> ALEEAPWPPPEGAFVGFVLSRK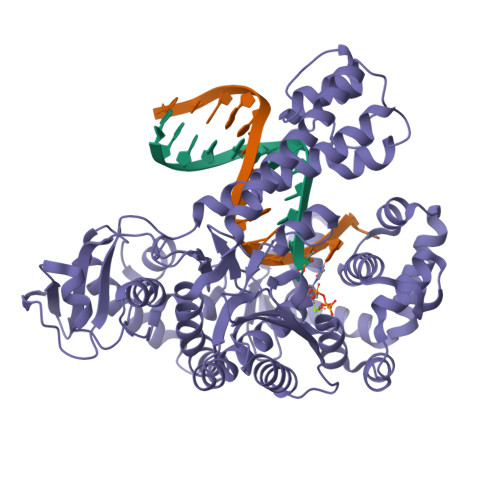EPMWADLLALAAARGGRVHRAPEPYKALRDLKEARGLLAKDLSVLALREGLGLPPGDDPMLLAYLLDPSNTTPEGVARRYGGEWTEEAGERAALSERLFANLWGRLEGEERLLWLYREVERPLSAVLAHMEATGVRLDVAYLRALSLEVAEEIARLEAEVFRLAGHPFNLNSRDQLERVLFDELGLPAIGKTEKTGKRSTSAAVLEALREAHPIVEKILQYRELTKLKSTYIDPLPDLIHPRTGRLHTRFNQTATATGRLSSSDPNLQNIPVRTPLGQRIRRAFIAEEGWLLVALDYSQIELRVLAHLSGDENLIRVFQEGRDIHTETASWMFGVPREAVDPLMRRAAKTINFGVLYGMSAHRLSQELAIPYEEAQAFIERYFQSFPKVRAWIEKTLEEGRRRGYVETLFGRRRYVPDLEARVKSVREAAERMAFNMPVQGTAADLMKLAMVKLFPRLEEMGARMLLQVHDELVLEAPKERAEAVARLAKEVMEGVYPLAVPLEVEVGIGEDWLSAK> GCGGAAGUAGUUCAGUGGUAGAACACCCGACAGACGAAGCGCUAAAACGUGGGAUUCUGUCGGGGGGUCGCGG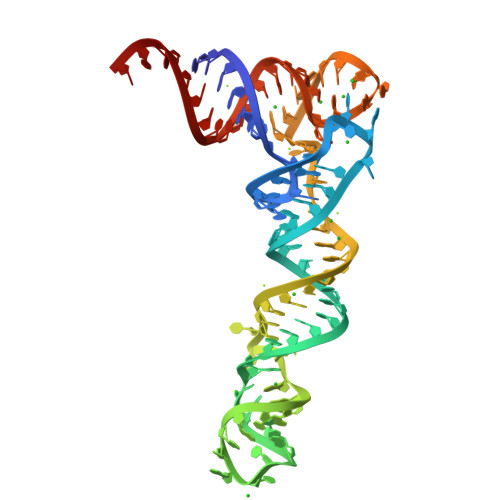GUUCGAGUCCCGUCUUCCGCUCCA>STAGKVIKCKAAVLWEEKKPFSIEEVEVAPPKAHEVRIKMVATGICRSDDHVVSGTLVTPLPVIAGHEAAGIVESIGEGVTTVRPGDKVIPLWTPQCGKCRVCKHPEGNFCLKNDLSMPRGTMQDGTSRFTCRGKPIHHFLGTSTFSQYTVVDEISVAKIDAASPLEKVCLIGCGFSTGYGSAVKVAKVTQGSTCAVFGLGGVGLSVIMGCKAAGAARIIGVDINKDKFAKAKEVGATECVNPQDYKKPIQEVLTEMSNGGVDF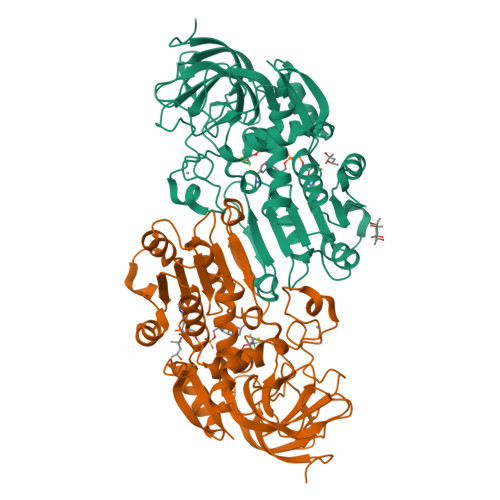SFEVIGRLDTMVTALSCCQEAYGVSVIVGVPPDSQNLSMNPMLLLSGRTWKGAIFGGFKSKDSVPKLVADFMAKKFALDPLITHVLPFEKINEGFDLLRSGESIRTILTF[2x]>MSESVTQQVFNFAVTKSQPFGGYVYSTNLTASTSSAVTSTQLTPLNLSITLGQITLSGNSLVIPATQIWYLTDAYVSVPDYTNITNGAEADGVILIYKDGVKLMLTTPLISSMSISNPARTHLAQAVKYSPQSILTMYFNPTKPATASTSYPNTVYFTVVVVDFSYAQNPARAVVSANAVM[42x];> MLSLDNYSYVHNITTQTNIDLSSQQTIHLASINGKGYIIFLRFFCEGSSACFTNVKFSVKANGLVLYSFRYIQLLELGQAIATAIPSSSQGFSTLLSNYN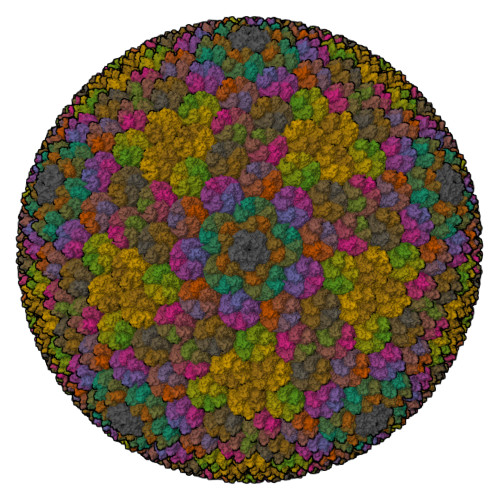VLISSPIGTLPQLTLYDSYDNRYGAMLQPAFPLPFVNTLSLDVDILPVSQSSYDPIPYSLNDNQISTNAPTGKGNISIEYLLYNCLV> ANIVGGIEYSINNASLCSVGFSVTRGATKGFVTAGHCGTVNATARIGGAVVGTFAARVFPGNDRAWVSLTSAQTLLPRVANGSSFVTVRGSTEAAVGAAVCRSGRTTGYQCGTITAKNVTANYAEGAVRGLTQGNACAGRGDSGGSWITSAGQAQ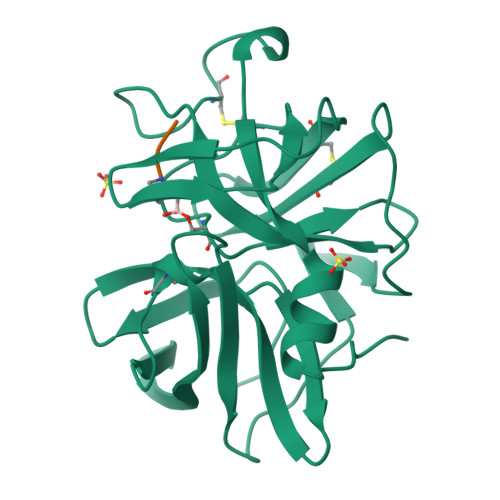GVMSGGNVQSNGNNCGIPASQRSSLFERLQPILSQYGLSLVTG;> XAAPA>MPVITVNTNVAEKSIP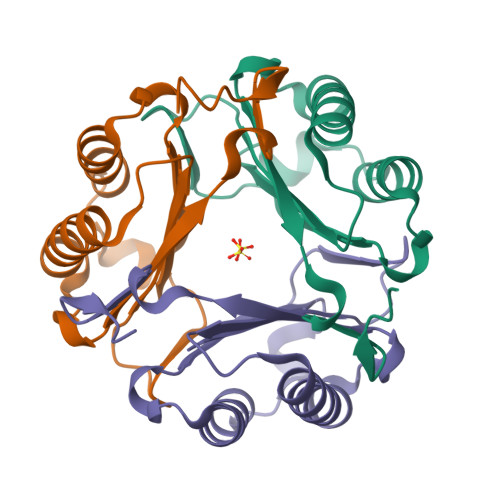VFFQAALTNMMTKALQKPKEVMFVDLRSGANIMMGGDRNPCVFATVECIGRLNPTSNLAMARDMEDMFIEHLNVRRERIVIRFIPVPALFCSFNGALHDVSIERDEYLEHHHHHH[12x]> SNAMFTINTKSQLPIYEQIVQKIKEQVVKGVLQEGEKILSIREFASRIGVNPNTVSKAY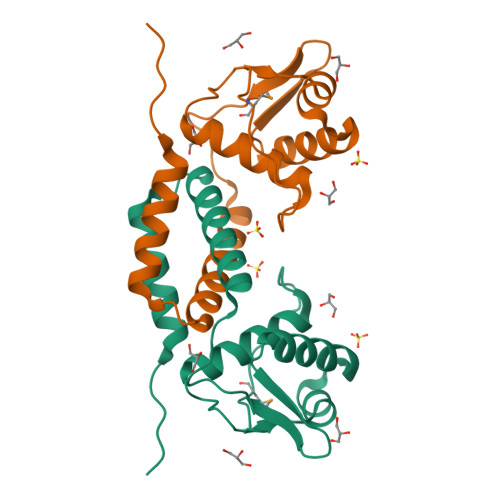QELERQEVIITVKGKGTFIANQTDKLSSPKKLAETRTKLKETILDLVYLGVNIEEIHKLADEYSQDIIGGDVVEG> 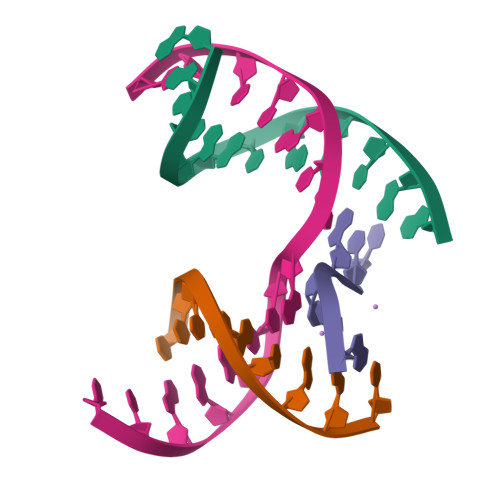GAACGACATTGA;> CGACGACTC;> TCATCG;> TCGAGTCAGTGTCGT> MDPIALQAGFDLLNDGRPETLWLGIGTLLMLIGTFYFIARGWGVTDKEAREYYAITILVPGIASAAYLAMFFGIGVTEVELASGTVLDIYYARYADWLFTTPLLLLDLALLAKVDRVTIGTLIGVDALMIVTGLIGALSKTPLARYTWWLFSTIAFLFVLYYLLTSLRSAAAKRSEEVRSTFNTLTALVAVLWTAYPILWIVGTEGAGVVGLGIETLAFMVLDVTAKVGFGFVLLRSRAILGETEAPEPSAGADASAAD

Archaerhodopsin-2 (aR2), the sole protein found in the claret membrane of Halorubrum sp. Aus-2, functions as a light-driven proton pump. Since the light-driven proton pump bacteriorhodopsin was discovered in the cell membrane of Halobacterium salinarum, a large number of proton-pumping rhodopsins have been found in diverse species, including archaea, eubacteria, fungi and algae. Although the structure of the proton-release pathway is highly conserved among proton-pumping archaeal rhodopsins, aR2 possesses the following peculiar structural features: (i) the motional freedom of the tryptophan residue that makes contact with the C13 methyl group of retinal is restricted, affecting the formation/decay kinetics of the L state, and (ii) the N-terminal polypeptide folds into an Ω-loop, which may play a role in organizing the higher-order structure.

In this study, we have applied the membrane-fusion method to prepare a novel three-dimensional crystal of aR2. This crystal is made up of membranous layers, in each of which the aR2 trimers are arranged on a hexagonal lattice. Compared with the previously reported crystal forms of aR2, the new crystal has several advantages: (i) it diffracts X-rays to a higher resolution, (ii) the problem of crystal twinning is avoided and (iii) the hexagonal array as seen in the native claret membrane is reconstituted in the crystal. In space group H32, one subunit of aR2 is contained in the asymmetric unit; i.e. the aR2 trimer is supposed to have perfect threefold symmetry. Specifically, a hydrocarbon chain (possibly squalene) is positioned at the centre of the trimer, breaking the threefold symmetry. Owing to these properties, the new crystal provided accurate structural information about functionally important residues. It is shown that two glutamates (Glu199 and Glu209) in the proton-release channel are separated by a very short distance (2.3 Å). The retinal chromophore bound to the ∊-amino group of Lys220aR2 in helix G adopts the all-trans configuration. Although most residues in the retinal-binding pocket are highly conserved in proton-pumping archaeal rhodopsins, Met145 in bR is replaced by phenylalanine (Phe150) in aR2.>[10x]QANLMRLK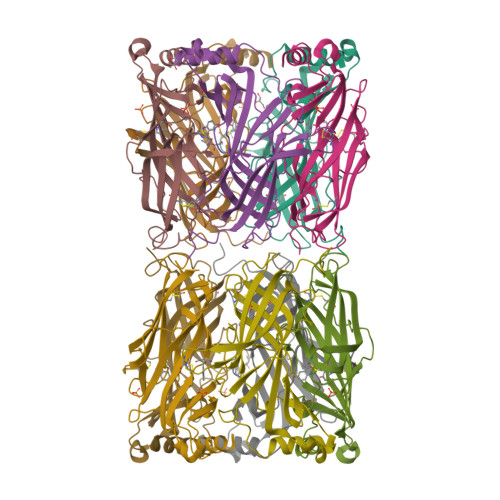SDLFNRSPMYPGPTKDDPLTVTLGFTLQDIVKVDSSTNEVDLVYWEQQRWKLNSLMWDPNEYGNITDFRTSAADIWTPDITAYESTRPVQVLSPQIAVVTHDGSVMFIPAQRLSFMCDPTGVDSEEGVTCALTFGSWVYSGFEIDLKTDTDQVDLSSYYASSKYEILSATQTRQVQHYSCCPEPYIDVNLVVKFRERRAGNGFF> SVRPWEFRKVIQAEYRERLPRNYELKHWKKPSKI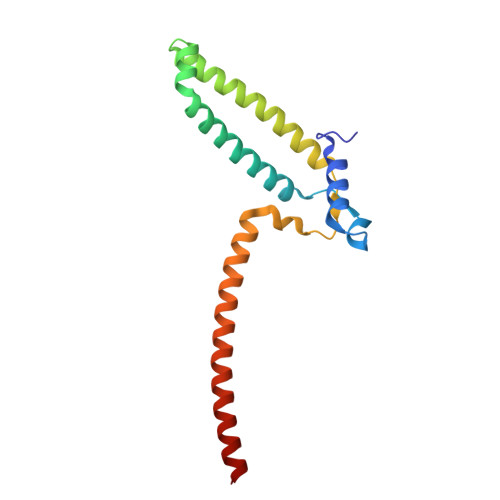MIGSILRLLETNTVSALDSVFEKYEKEMNQMTHGDNNEVKRIYSKKERLLEIILTKIKKKLRQAKFPSRISERDLDIEYIYSKRQFIQNRYSQELQNNERLEAILSREQNLLEETRKL OmIA, α-conotoxin purified from Conus omaria, is an α4/7-conotoxins that competitively antagonises α7 nAChRs. nAChRs are prototypical ligand-gated ion channels found in the central and peripheral nervous system, and recently in other biological systems such as in immune system, muscles, skin and lung. Among different nAChRs subtypes, the homopentameric α7 nAChR is one of the most abundant nAChRs in the nervous system and also in many non-neuronal cells. We determined the co-crystal structure of OmIA with Lymnae stagnalis acetylcholine binding protein (Ls-AChBP) that identified His5, Val10 and Asn11 as key determinants for the high potency of OmIA at α7 nAChRs.

The structure of OmIA and Ls-AChBP was solved at 2.47 Å resolution. A tight homopentameric ring assembly of subunits was observed for the OmIA/Ls-AChBP complex, where OmIA occupied all five binding pockets located between two adjacent protomers. The N and C termini of bound OmIA orientated towards the top and bottom of the LBP, respectively, with the central helix abutting into the binding pocket. Structural superimposition with the HEPES/Ls-AChBP structure revealed that the C-loop of Ls-AChBP moved out a comparable distance (9.3 ± 0.4 Å from the Cys187 Cα atom) and had a similar backbone orientation to previously characterised co-crystal structures. Each of the five bound OmIA molecules interacted in a similar orientation (RMSD = 0.090 ± 0.005 Å) at the interface between two adjacent Ls-AChBP protomers that formed the principal and complementary binding sides. Most interactions on the principal side were between His5 and Ala7 of OmIA and C-loop residues Tyr185–Tyr192, as well as interactions between the disulfide bridge of OmIA and the vicinal disulfide Cys188-Cys189 of Ls-AChBP. His5 resided in a pocket formed by aromatic side-chain residues, specifically Tyr89, Tyr192 and Tyr185, and formed hydrogen bond with Tyr89 and the backbone oxygen of Glu193. On the complementary side, OmIA_Asn9 interacted with a surface comprising charged residue Lys34, polar residues Ser32, Gln55, Tyr164, and hydrophobic residue Met114, in which hydrogen bonds were seen between Asn9/Gln55 and Asn9/Tyr164. OmIA_Val10 interacted in a pocket formed by Thr144 on the principal side and Arg104, Leu112 and Met114 on the complementary side of Ls-AChBP. The surface interacting with OmIA_Asn11 in the co-crystal structure comprised mostly polar and charged residues from both the principal (Thr144, Glu149 and Tyr192) and complementary faces of each subunit interface (Gln73 and Arg104), where hydrogen backbone were seen between Asn11/Thr144 and Asn11/Gln73.

>[5x]LDRADILYNIRQTSRPDVIPTQRDRPVAVSVSLKFINILEVNEITNEVDVVFWQQTTWSDRTLAWNSSHSPDQVSVPISSLWVPDLAAYNAISKPEVLTPQLARVVSDGEVLYMPSIRQRFSCDVSGVDTESGATCRIKIGSWTHHSREISVDPTTENSDDSEYFSQYSRFEILDVTQKKNSVTYSCCPEAYEDVEVSLNFRKKGRSEIL;>GCCSHPACNVNNPHICGX[5x]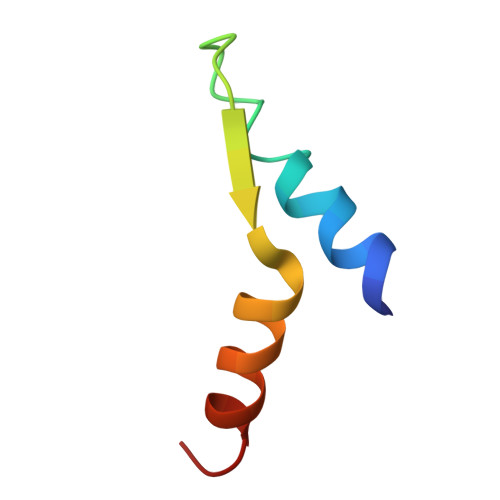> TITEWSVNMYNHLRGTGEDENILFSPLSIALAMGMMELGA>MIFQQLFESSSSTYTYLLGCPITKTAVLIDPVLETVERDISILNALGLTLRYTLETHIHADHLSGGYQLRQRTGCLIALPAIEQLPCADIGIEEGTPLCVGEVQIHPLYTPGHTSSHHAYYVDTGTHLMLFSGDALLIDACGRTDFQAGNAGQLYDSIQHKLFTLPNETLVYPGHDYEGRFISSIAQEKQRNPRLSNNKSKQAFIELMNGLKTPNPRKMAFAVPSNKQCGMCPPNIFEEYQQLCETLV[2x]

Oxidation of sulfane sulfur can also be carried out by persulfide dioxygenase (PDO) from the superfamily of metallo-β-lactamase enzymes. However, PDO does not oxidize elemental sulfur directly because its direct substrate is glutathione persulfide (GSSH). Here, we report the first structure of a recombinant PDO obtained for a representative from a group of colorless filamentous sulfur bacteria, Beggiatoa leptomitoformis, and provide a comparative structural and biochemical characterization with known PDOs. Thus, it was shown that B. leptomitoformis uses PDO to oxidize endogenous sulfur.

The B. leptomitoformis PDO structure reveals dimeric organization and contains an αββα metal-binding fold with two central mixed β-sheets, each containing six strands, surrounded on both sides by helices. In the B. leptomitoformis PDO structure, 14 residues from the C-terminus are not visible, which indicates the mobility of this region. Thus, in PDO from B. leptomitoformis, the interface area between monomers is not extensive (997 Å2), as also seen in the similar area in the structure of PDO from A. thaliana. There are 10 hydrogen bonds involved in the formation of contacts between B. leptomitoformis PDO monomer molecules, and there is a hydrophobic interaction. In the active site of PDO from B. leptomitoformis, the residues of the first coordination sphere of the iron ion (His57, His113, Asp134, and three water molecules) are identical to those of other type I PDO structures. The substrate in the active site of the B. leptomitoformis PDO can be coordinated by an iron ion, Arg194, Tyr177, and Asp61. The amino acid residues of the putative substrate-binding pocket of the B. leptomitoformis PDO, as in other type I PDOs, form two walls, one structurally rigid, conserved wall formed by, among others, Arg194 and Tyr177, and a second wall opposite, a structurally mobile wall formed by two loops. However, in the PDO of B. leptomitoformis, Phe146 makes a hydrophobic contribution to the active site surface, while the charged group of Gln147 participates in the formation of the dimer interface. The second coordination sphere of the iron ion in the PDO of B. leptomitoformis differs from other known type I PDO structures by a single residue (His117), with His replaced by Cys in hETHE1 and BpPRF or Ser in MxPDOI. The His117 side group, unlike cysteine and serine in the corresponding position, displaces water molecules located in the internal cavity of the enzyme, which can stabilize the hydrogen bonding network near the active center and affect the enzyme activity.> MISHIQTNNNMPPGVQKNFKTFGVPLESLIEFEQDMVPAIVRQCIYVIDKFGLDQEGIYRKSANVLDVSKLKEEIDKDPANISMILPSKPHSDSDIYLV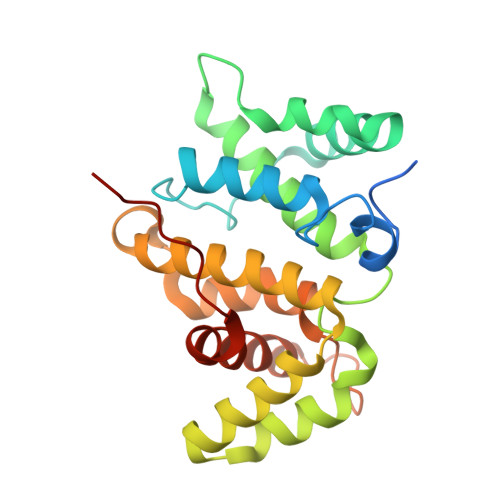GSLLKTFFASLPDSVLPKALSSEIKVCLQIEDPTTRKNFMHGLIYNLPDAQYWTLRALVFHLKRVLAHEAQNRMNLRALCIIWGPTIAPANPDDANDVNFQIMAMEVLLEVSDQAFEPELEHHHHHH>[4x]MQIYHTDVLCIGGALAGERVAVEASMAGLKTIMLSLVPPRRSHSSAAQGGMQAALGNAIMGDGDSPDVHFADTVKGSDWGCDQEVARIFADTAPIVMREVAHWGVPWNR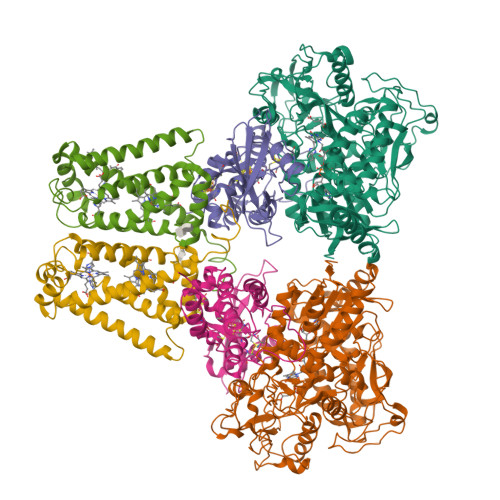VVPGKHTYYKGGKPFEAEEKAEKAGLIHARAFGGTAAWRTCYTADGTGRSVLNTLDTKCLQYGVTVHDRMQAEALIHDGGNCLGCIARCLRTGELVAYLATSTLIATGGYGRIYKATTNAVICDGGGQIIALDTGLVPMGNMEAVQFHPTGTVPTDILVTEGCRGDGGTLLDVNQYRFMPDYEPDKAQLASRDVVSRRMTEHMRKGLGVKSPYGDHLWLDIRHLGEKHITTKLREVYDICTNFLGVNPIHQLIPVRPTHHYSMGGVRTNRDGAAYGLKGLFSAGESACWDMHGFNRLGGNSLAETVVAGRYIGERMVEFTKGATPSFGMQYVEDAHKKVQERITDIVTGRKGKENTFKIRDEMHDIMMEGVGIFRNGTDLQKAVNKLEELYDRSQKISLSSACKGMNPELSTALRIRGMLKLAQCTAYGALDRTESRGAHTREDFPERNDKEWLNRTLSYWKEGASMPTLEYEEASPYYEMPPGDRGYGGGVTIANELPPEKFVIPEAAKENLKKAKL;>[4x]MNRMLTLNIFRYNPLDPDSQPRMQTFTVQEYDSMTLFIALTQIRDEKDPTLKVDFCCRAGICGSCAMVINGRPGLACHTQTKDLPAEITLHPLPFFQLLGDLSVDTGSWFRKTGLQIEAWCHSDDKAFDPTADEMRMDNDLANEIFELDRCIECGCCVAACGTARMRTDFLGAVSIMRVARFYLDPRDKRSEDDYYDVIGNDQGVFGCMGLLACEDVCPKGIPLQDQLGIMRRMMAMHSVKGVLPRPLIETIKKKGCCHAHAQS;>MNASTITLHVPQRSKIAGRMDFFQMVSGALLILFLWAHMMLVSSVILSPSLMNGIAWFFEATYMAQIGGPAVFVLMVVHFILAARKMPFKQDEWKTFRVHACMLHHKDTTMWVVQVISAIFILVLGAVHMFVVLTDLPITAAKSAARLQSGWLYLYLVLLPLAELHVGVGFYRIGVKYGFVGRNKRKWFQKTENLMMIGFITIGLLTLVRFMLLNIQG[4x]> MRVRLSKTLAGILRHHPGRYGVRL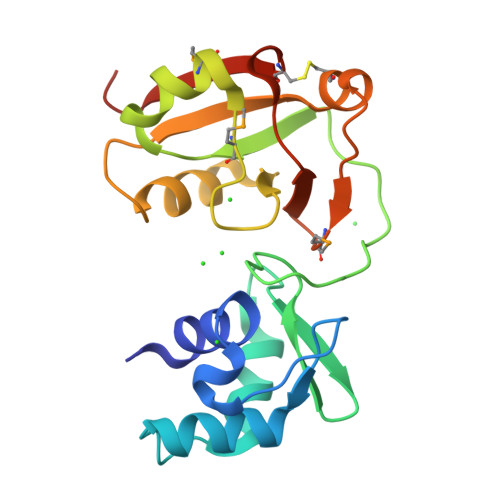TREGWARVSEVVEGLRKAGWSWVEEWHIVGVALHDPKGRYELRNGEIRARYGHSIPVNVEPLPGEPPPILYHGTTEEALPLIMERGIMRGRRLKVHLTSSLEDAVSTGRRHGNLVAVLLVDVECLRRRGLKVERMSKTVYTVDWVPPECIAEVRRESLGRSL>AELVSDKALESAPTVGWASQNGFTTGGAAATSDNIYIVTNISEFTSALSAGAEAKIIQIKGTIDISGGTPYTDFADQKARSQINIPANTTVIGLGTDAKFINGSLIIDGTDGTNNVIIRNVYIQTPIDVEPHYEKGDGWNAEWDAMNITNGAHHVWIDHVTISDGNFTDDMYTTKDGETYVQHDGALDIKRGSDYVTISNSLIDQHDKTMLIGHSDSNGSQDKGKLHVTLFNNVFNRVTERAPRVRYGSIHSFNNVFKG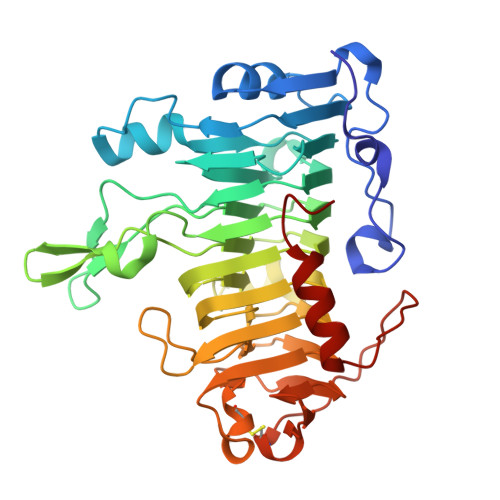DAKDPVYRYQYSFGIGTSGSVLSEGNSFTIANLSASKACKVVKKFNGSIFSDNGSVLNGSAVDLSGCGFSAYTSKIPYIYDVQPMTTELAQSITDNAGSGKL[2x]> AIDPFTMAKDFSKTSDEDLAKMAGVVAPQDIVDYTKELKK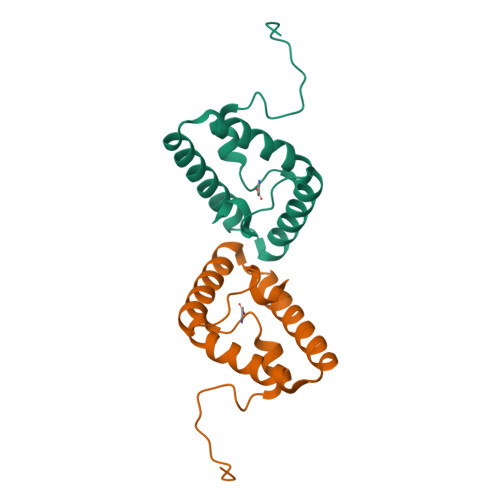RMEKMPEDKRKAFHKQLHEYATKNTDKMTVADFEARQKAVKEALKKGNMEDMDDDFGLRS1-BROMOPENTANE 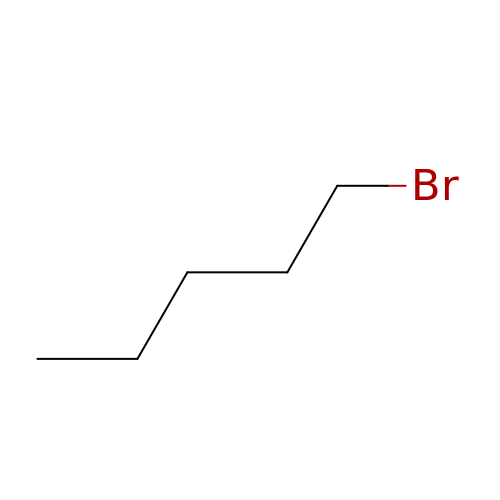| C5 H11 Br | YZWKKMVJZFACSU-UHFFFAOYSA-N methyl (4aS,6aR,6bS,8aR,12aS,14aS,14bS}-11-cyano-2,2,6a,6b,9,9,12a-heptamethyl-10,14-bis(oxidanylidene)-1,3,4,5,6,7,8,8a,14a,14b-decahydropicene-4a-carboxylate 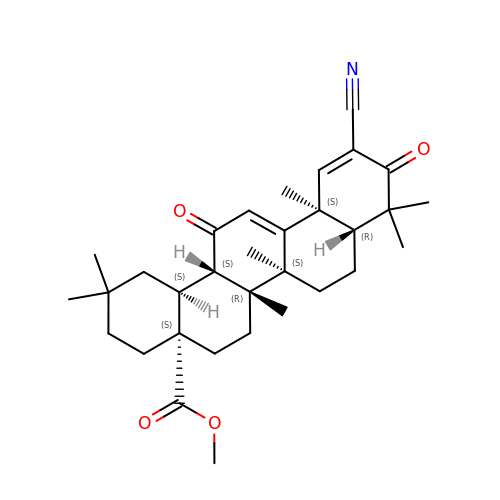| C32 H43 N O4 | WPTTVJLTNAWYAO-IIHRHBSVSA-N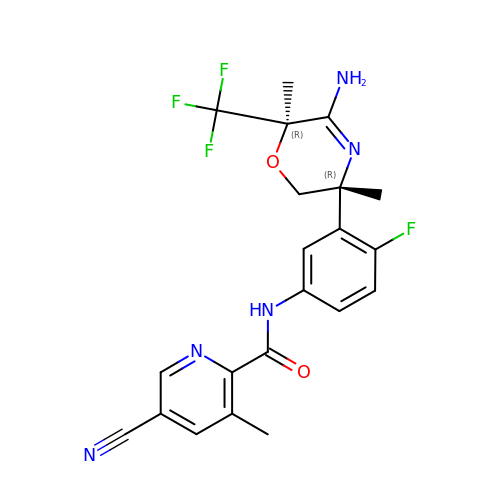~{N}-[3-[(3~{R},6~{R})-5-azanyl-3,6-dimethyl-6-(trifluoromethyl)-2~{H}-1,4-oxazin-3-yl]-4-fluoranyl-phenyl]-5-cyano-3-methyl-pyridine-2-carboxamide | C21 H19 F4 N5 O2 | BQFHTVUWPJXLOW-VQTJNVASSA-N>AKSVVSHSLTTLGVEVSKPPPQHDKIEASEPSFPLHESILKVVEEEWQQIDRQLPSVACRYPVSSIEAARILSVPKVDDEILGFISEATPAAATQASSTESCDKHLDLALCRSYEAAASALQIAAHTAFVAKSLQADISQAAQIINSDPSDAQQALRILNRTYDAASYLCDAAFDEVRMSACAMGSSTMGRRYLWLKDCKISPASKNKLTVAP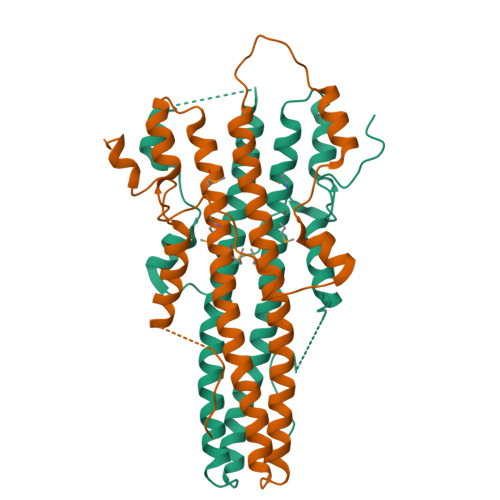FKGGTLFGGEVHKVIKKRGNKQ[2x]> HHHHHHEHTWPDKGSLYIATTHTQARYAL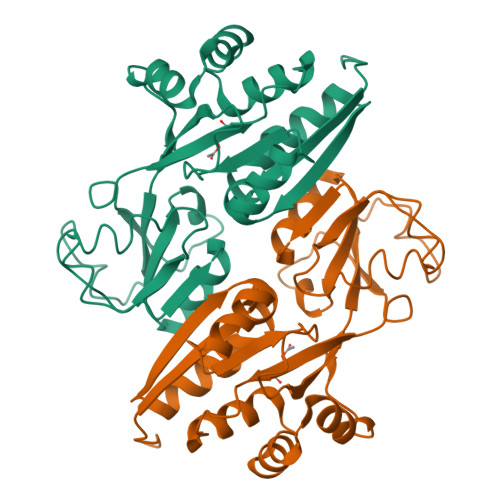PGVIKGFIERYPRVSLHMHQGSPTQIAEAVSKGNADFAIATEALHLYDDLVMLPCYHWNRSIVVTPDHPLAATSSVTIEALAQYPLVTYTFGFTGRSELDTAFNRAGLTPRIVFTATDADVIKTYVRLGLGVGVIASMAVDPLADPDLVRIDAHDIFSHSTTKIGFRRSTFLRSYMYDFIQRFAPHLTRDVVDTAVALRSNEEIEAMFQDIKLPEK Protein stability can be fine‐tuned by modifying different structural features such as hydrogen‐bond networks, salt bridges, hydrophobic cores, or disulfide bridges. Among these, stabilization by salt bridges is a major challenge in protein design and engineering since their stabilizing effects show a high dependence on the structural environment in the protein, and therefore are difficult to predict and model. In this work, we explore the effects on structure and stability of an introduced salt bridge cluster in the context of three different de novo TIM barrels. The results show that despite the similarities in protein fold, the salt bridge clusters differently influence the structural and stability properties of the de novo TIM barrel variants depending on the structural background where they are introduced.

The salt bridge variants exhibit similar thermostability in comparison with their parental designs but important differences in the conformational stability at 25°C can be observed such as a highly stabilizing effect for two of the proteins but a destabilizing effect to the third. Analysis of the formed geometries of the salt bridge cluster in the crystal structures show either highly ordered salt bridge clusters or only single salt bridges. Rosetta modeling of the salt bridge clusters results in a good prediction of the tendency on stability changes but not the geometries observed in the three‐dimensional structures.

> MDKDEAWKQVEQLRREGATRIAYRSDDWRDLKEAWKKGADILIVDATDKDEAWKQVEQLRREGATEIAYRSDDWRDLKEAWKKGADILIVDATDKDEAWKQVEQLRREGATRIAYRSDDWRDLKEAWKKGADILIVDATDKDEAWKQVEQLRREGATEIAYRSDDWRDLKEAWKKGADILIVDATGLEHHHHHH>[2x]MIKKAVLPVAGLGTRFLPASKSIPKEMVTVVDRPAIEYVVREAVEAGIEQIILVTHSSKASIENYFDRNFELETTLEQKKKFDLLAEITQIVPEHVSVISVRQPQPLGLGHAVLCAKSVVGEDDFAVLLPDVLVKDGSGQNDLSRMISRYNSSQAAQIMVEAVPDH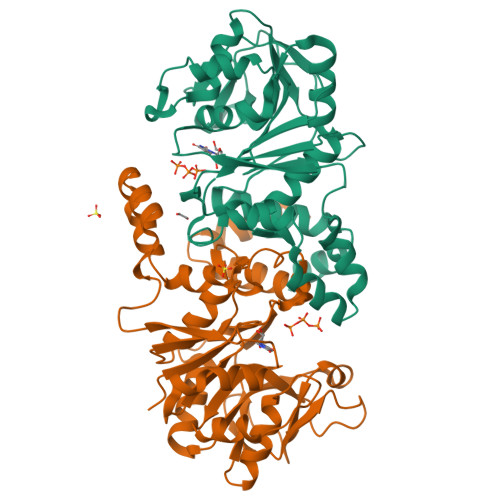LVDQYGIVDVAQSPNEGESIAMQGIVEKPPVGAAPSNLSVVGRYVLPAKIMQLLENTPKGAGNEIQLTDAIAMLQDTDTVEAYRMQGQTFDCGSKLGYLKAVLHYGLEHPKLGMEFKQLILELK Heat shock factor 1 (HSF1) and 2 (HSF2) play distinct but overlapping regulatory roles in maintaining cellular proteostasis or mediating cell differentiation and development. Upon activation, both HSFs trimerize and bind to heat shock elements (HSEs) present in the promoter region of target genes. HSFs recognize and bind HSEs through the DBD, which is the most conserved and only structurally characterized domain. Here, we present co-crystal structures of human HSF1 and HSF2 trimers bound to DNA, which reveal a triangular arrangement of the three DNA-binding domains (DBDs) with protein-protein interactions largely mediated by the wing domain.

Previous biochemical studies have shown that HSF1 and HSF2 bind to a two-site tail-to-tail HSE with higher affinity than to a head-to-head counterpart (Tateishi et al., 2009), but the structural basis for this difference is not well understood owing to the lack of head-to-head structures. To address this question, we first determined two structures: HSF2-DBD (residues 7–112) bound to a 12-bp oligonucleotide and HSF1-DBD (residues 15–120) bound to a 14-bp oligonucleotide at resolutions 1.7 and 2.0 Å. The DNA molecules present in both crystals comprised blunt-ended head-to-head sequences but packed with different orientations in the crystal lattice: head-to-tail versus head-to-head in the HSF2 and HSF1 structures, respectively. All base pairs were well defined in electron density except for an invisible terminal pair present in the HSF1 structure. Similar to the reported structures containing tail-to-tail HSEs, all sequence-specific interactions occur in the major groove and are principally donated by the bidentate hydrogen bonds between an invariant Arg residue (Arg63 in HSF2 or Arg71 in HSF1) and the guanine in the GAA triplet. The dimerization is weakly maintained by contacts between the short turns present in the helix-turn-helix motif, where only one residue (Lys54 in HSF2 and Lys62 in HSF1) is involved in forming a 2-fold symmetric pair of hydrogen bonds. Notably, the wing domain in both DBDs remains unstructured in our structures, but obviously stretched away from the dimer interface to opposite directions. In comparison with HSF2, one HSF1 monomer slightly moved away along the DNA axis. The relative movement reflects a more extended binding manner of the HSF1 dimer, or in other words, HSF1 occupying a longer DNA segment than HSF2.

>[2x]GHHHHHHVPAFLTKLWTLVSDPDTDALICWSPSGNSFHVFDQGQFAKEVLPKYFKHNNMASFVRQLNMYGFRKVVHIEQGGLVKPERDDTEFQHPCFLRGQEQLLENIKRKVT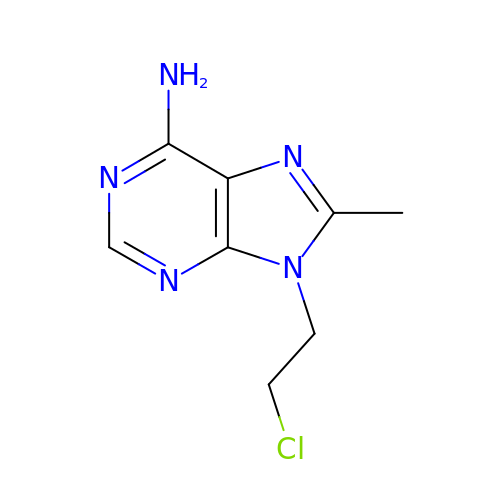9-(2-chloroethyl)-8-methyl-purin-6-amine | C8 H10 Cl N5 | XOAPLONMSUKXAM-UHFFFAOYSA-N> MGSADAQSFLNRVCGVSAARLTPCGTGTSTDVVYRAFDIYNDKVAGFAKFLKTNCCRFQEKDEDDNLIDSYFVVKRHTFSNYQHEETIYNLLKDCPAVAKHDFFKFRIDGDMVPHISRQRLTKYTMADLVYALRHFDEGNCDTLKEILVTYNCCDDDYFNKKDWYDFVENPDILRVYANLGERVRQALLKTVQFCDAMRNAGIVGVLTLDNQDLNGNWYDFGDFIQTTPGSGVPVVDSYYSLLMPILTLTRALTAESHVDTDLTKPYIKWDLLKYDFTEERLKLFDRYFKYWDQTYHPNCVNCLDDRCILHCANFNVLFSTVFPPTSFGPLVRKIFVDGVPFVVSTGYHFRELGVVHNQDVNLHSSRLSFKELLVYAADPAMHAASGNLLLDKRTTCFSVAALTNNVAFQTVKPGNFNKDFYDFAVSKGFFKEGSSVELKHFFFAQDGNAAISDYDYYRYNLPTMCDIRQLLFVVEVVDKYFDCYDGGCINANQVIVNNLDKSAGFPFNKWGKARLYYDSMSYEDQDALFAYTKRNVIPTITQMNLKYAISAKNRARTVAGVSICSTMTNRQFHQKLLKSIAATRGATVVIGTSKFYGGWHNMLKTVYSDVENPHLMGWDYPKCDRAMPNMLRIMASLVLARKHTTCCSLSHRFYRLANECAQVLSEMVMCG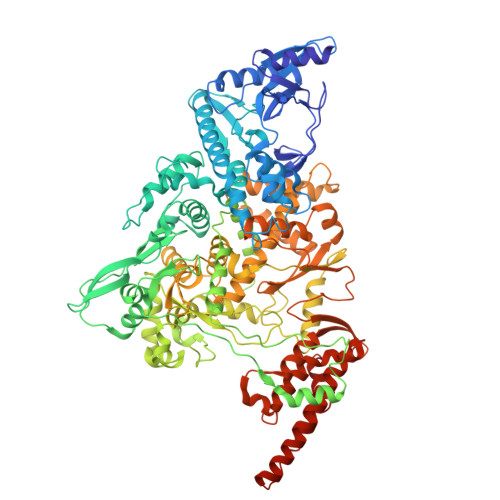GSLYVKPGGTSSGDATTAYANSVFNICQAVTANVNALLSTDGNKIADKYVRNLQHRLYECLYRNRDVDTDFVNEFYAYLRKHFSMMILSDDAVVCFNSTYASQGLVASIKNFKSVLYYQNNVFMSEAKCWTETDLTKGPHEFCSQHTMLVKQGDDYVYLPYPDPSRILGAGCFVDDIVKTDGTLMIERFVSLAIDAYPLTKHPNQEYADVFHLYLQYIRKLHDELTGHMLDMYSVMLTNDNTSRYWEPEFYEAMYTPHTVLQHHHHHHHHHH>MGSKSFLTEQQIKILRLRARGLKQSEIAELLGTSRANISILERRALEKIEKARNTITIWEQINSKISVEVRKGEDIFTVPDKLFKKADELQIKVPYSTAEIIAFLVEHAPISDRIAKRDFTLFLDARDRLRISECLLEEFDEIGKQHHHHHH[2x]

Thermococcus onnurineus NA1, a hyperthermophilic carboxydotrophic archaeon, produces H2 through CO oxidation catalyzed by proteins encoded in a carbon monoxide dehydrogenase (CODH) gene cluster. TON_1525 with a DNA-binding helix-turn-helix (HTH) motif is a putative repressor regulating the transcriptional expression of the codh gene cluster. Monomeric TON_1525 adopts a novel ‘eighth note’ symbol-like fold (referred to as ‘eighth note’ fold regulator, EnfR), and the dimerization mode of EnfR is unique in that it has no resemblance to structures in the Protein Data Bank. According to footprinting and gel shift assays, dimeric EnfR binds to a 36-bp pseudo-palindromic inverted repeat in the promoter region of the codh gene cluster, which is supported by an in silico EnfR/DNA complex model and mutational studies revealing the implication of N-terminal loops as well as HTH motifs in DNA recognition.

We determined the 2.8 Å resolution crystal structure of the wild-type TON_1525. There are two monomers in the asymmetric unit of the wild-type TON_1525 crystals, which is compatible with our demonstration that TON_1525 is a dimeric protein in solution. The structures of the two monomers are virtually identical; their structures are superposed with the root mean square (r.m.s.) deviation of 0.490 Å for all Cα atoms. Monomeric structure of TON_1525 resembles an ‘eighth note (♩)’ symbol in that it can be divided into three parts: a flag, a straight stem and a note-head (hereafter referred to as ‘eighth note’ fold regulator, EnfR). The flag part contains two N-terminal α1 and α2 helices (residues 1–34), the stem part is a long α3 helix (residues 35–62) and the note-head corresponds to the C-terminal α+β domain (residues 63–146) in which a three-stranded antiparallel β-sheet (↑β1-↓β2-↑β3) is sandwiched by the stem helix (α3) on one face and two C-terminal helices (α4 and α5) on the other face. The dimerization of EnfR is mediated mainly by the flag and stem helices with a contact area of ∼2300 Å2, covering one-third of the molecular surface of a monomer. The long stem helices from two monomers form antiparallel X-shaped cross interactions. In the dimeric structure, two α2-turn-α3 HTH motifs are ∼35.8 Å apart from each other (using the Cα of Glu42 as a reference point). In the wild-type dimer, the side chain hydroxyl group of Thr55 in a monomer is hydrogen-bonded to the backbone –NH group of Phe6 in another monomer, which directs the N-6 region to extend out of the main body. Two benzyl side chains of Phe6 in the N-6 regions of two monomers form π–π stacking interaction to stabilize the observed conformation of the N-6 region.>MKIKIGGKDMRTTDMKGIYSALLVSFDKEGNINEKGLRQIIRHNIDVCKVDGLYVGGSTGENFMLSTDEKKRIFEIAKDEVKEEIKLIAQVGSVNLKEAVELAKFTTDLGYDAISAVTPFYYKFDFEEIKHYYNTIINSVDNRLIIYSIPFLTGVDMSLDQFGELFENEKIIGVKFTAADFYLLERMRKTFPNKLIFAGFDEMMLPATVLGVDGAIGSTFNVNGVRARQIFELTKNEKISEALEVQHVTNDLITDILGNGLYQTIKLLLEEQGVEAGYCRQPM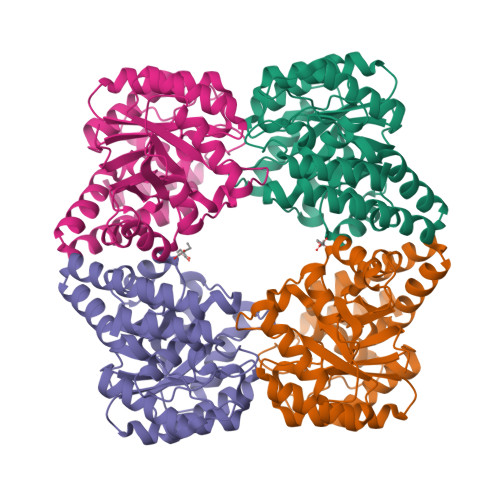KEATDEMKSRAKEIYRKYF[8x]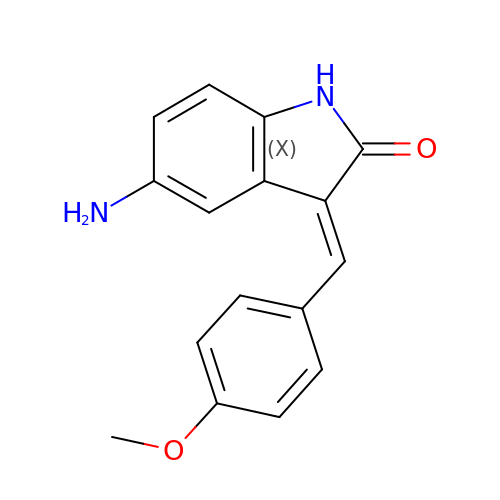(3Z)-5-AMINO-3-[(4-METHOXYPHENYL)METHYLIDENE]-1,3-DIHYDRO-2H-INDOL-2-ONE | C16 H14 N2 O2 | DYCBCUFDDRQCID-ZSOIEALJSA-N> SWLLRLFESKLFDISMAISYLYNSKEPGVQAYIGNRLFCFRNEDVDFYLPQLLNMYIHMDEDVGDAIKPYIVHRCRQSINFSLQCALLLGAYSSDMHISTQRHSRGTKLRKLILSDELKPAHRKRELPSLSPAPDTGLSPSKRTHQRSKSDATASISLSSNLKRTASNPKVENEDEELSSSTESIDNSFSSPVRLAPER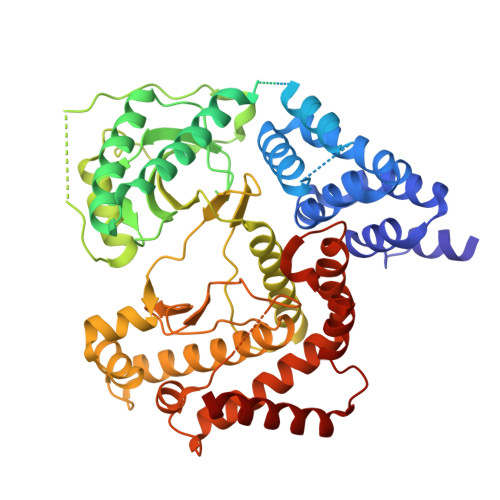EFIKSLMAIGKRLATLPTKEQKTQRLISELSLLNHKLPARVWLPTAGFDHHVVRVPHTQAVVLNSKDKAPYLIYVEVLECENFDTTSVPARIPENRRDPEDPSAVALKEPWQEKVRRIREGSPYGHLPNWRLLSVIVKCGDDLRQELLAFQVLKQLQSIWEQERVPLWIKPYKILVISADSGMIEPVVNAVSIHQVKKQSQLSLLDYFLQEHGSYTTEAFLSAQRNFVQSCAGYCLVCYLLQVKDRHNGNILLDAEGHIIHIDFGFILSSSPRNLGFETSAFKLTTEFVDVMGGLDGDMFNYYKMLMLQGLIAARKHMDKVVQIVEIMQQGSQLPCFHGSSTIRNLKERFHMSMTEEQLQLLVEQMVDGSMRS> MLELLPTAVEGVSQAQITGRPEWIWLALGTALMGLGTLYFLVKGMGVSDPDAKKFYAITTLVPAIAFTMYLSMLLGYGLTMVPFGGEQNPIYWARYADWLFTTPLLLLGLALLVDADQGTILALVGADGIMIGTG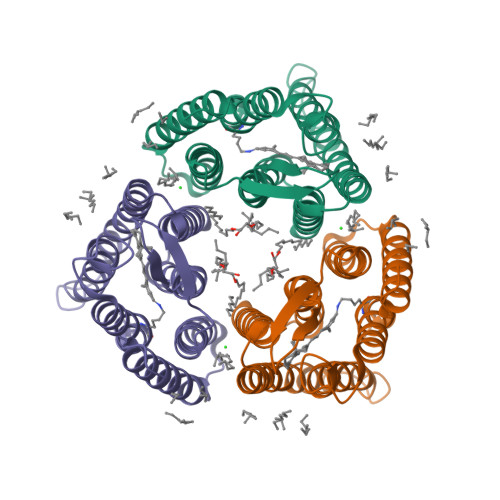LVGALTKVYSYRFVWWAISTAAMLYILYVLFFGFTSKAESMRPEVASTCKVLRNVTVVLWSAYPVVWLIGSEGAGIVPLNIETLLFMVLDVSAKVGLGLILLRSRAIFGEAEAPEPSAGDGAAATSD>[2x]MNIHEWQSKQLIQKYGGRAQSGEVAFSPERSRDIAKKLWNQFPGCKFVVKAQVL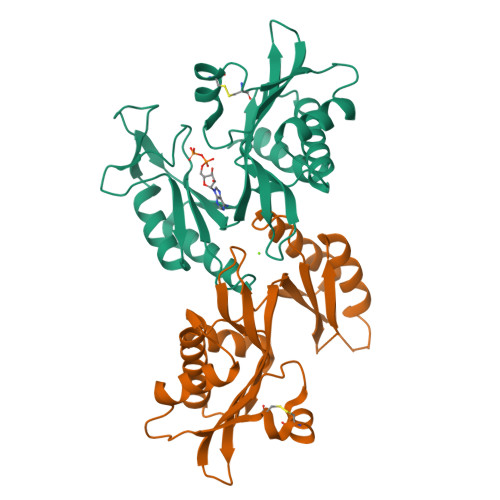AGGRGKGHWEHGMQGGVKLAKTPEEVYEIANEMIGHKLITKQTGAKGINCNKVMVCGAVKILKEFYLSILLDRAMGCPVIIATSQGGMGIEEVAQKCPECLFKVPISVKNGPTNEQLVKLAKDLGLEGDLVQDCVDNVKALYQVFDKCDSTMVEINPLGVIETPTDEKVICCFDAKIAFDKDAAFGLEHHHHHHHH> PVVNRGQGWAYEPMSTRTVAAWI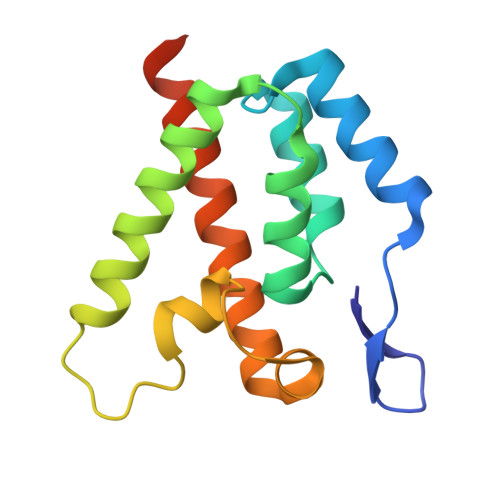RQTGEKGLTSPETITYWGLISQDLSSREQVQLLEVVPGLQADKDMLGAYLEERAREWDAQPQQPLPYTSAHIRGLTGDQAFAISAQGREAAQVFRAWITQGLMNLAQLRAPLEHHHHHH>[2x]MGSSHHHHHHQGYSNPVIPGFHPDPSVCKAGDDYYLVNSSFQYFPGVPLFHSKDLVHWEQIGNCLTRPSQLDLTNANSGSGIFAPTIRYNDGVFYMITTNVSGKGNFLVHTTDPRSEWSEPVWLEQGGIDPSLYFEDGKCFMVSNPDGYINLCEIDPMTGKQLSSSKRIWNGTGGRYAEGPHIYKKDGWYYLLISEGGTELGHKVTIARSRYIDGPYQGNPANPILTHANESGQSSPIQGTGHADLVEGTDGSWWMVCLAYRIMPGTHHTLGRETYLAPVRWDKDAWPVVNSNGTISLKMDVPTLPQQEMKGRPERIDFKEGKLSPEWIHLQNPEAKNYIFTKDGKLRLIATPVTLSDWKSPTFVALRQEHFDMEASAPVVLQKAGVNDEAGISVFMEFHSHYDLFVRQDKDR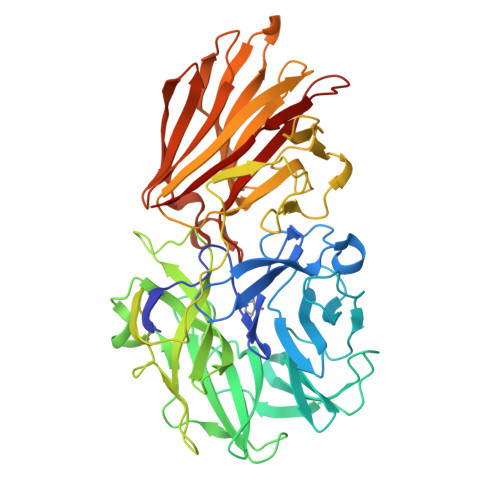KRSVGLRYKLGEITHYAKEVSLPTDGEVELVVKSDINYYYFGYKVNGIYHDLGKMNTRYLSTETAGGFTGVVLGLYITSASKDSKAYADFEYFKYKGKPGENK>[6x]MCGRFLRRLLAEESRRSTPVGRLLLPVLLGFRLVLLAASGPGVYGDEQSEFVCHTQQPGCKAACFDAFHPLSPLRFWVFQVILVAVPSALYMGFTLYHVIWHWELSGKGKEEETLIQGREGNTDVPGAGSLRLLWAYVAQLGARLVLEGAALGLQYHLYGFQMPSSFACRREPCLGSITCNLSRPSEKTIFLKTMFGVSGFCLLFTFLELVLLGLGRWWRTWKHKSSSSKYFLTSESTRRHKKATDSLPVVETKEQFQEAVPGRSLAQEKQRPVGPRDA

Connexin family proteins assemble into hexameric channels called hemichannels/connexons, which function as transmembrane channels or dock together to form gap junction intercellular channels (GJIChs). Human Cx31.3/GJC3, which is expressed in oligodendrocytes of the central nervous systems, does not form intercellular channels. We determined the cryo–electron microscopy structures of human connexin 31.3 (Cx31.3)/GJC3 hemichannels in the presence and absence of calcium ions and with a hearing-loss mutation R15G at 2.3-, 2.5-, and 2.6-Å resolutions, respectively. We also found that the hemichannel has a pore with a diameter of ~8 Å and selectively transports chloride ions.

Six NTHs in the hemichannel are placed at the cytoplasmic entrance, whereas those in GJIChs are at the inner surface of the pore. The entrance-covering conformation appears to be stabilized mainly by intramolecular hydrophobic interactions of F5 and L9 in NTH, with T95, L96, V99, I100, and W103 in TM2. With this structure, we analyzed the solvent-accessible pore diameters along the pore axis and found that NTHs form the smallest pore with a diameter of ~8 Å, which is smaller than those of Cx26 (10 Å) and Cx46/50 (11 Å) GJICh structures. We identified long chains of map density on the hydrophobic surface, which likely correspond to lipid or detergent molecules. A strong density blob is located next to R144 in a deep hydrophilic pocket at the boundary of cytoplasmic and transmembrane regions, which spatially fit well at the head group of phosphatidylethanolamine (PE). In our putative PE-bound model, the phospho and amino groups of PE interact with the guanidino group of R144 and the carboxyl group of E13, respectively. In the Ca2+-free state, the tunnel is occupied by six water molecules (W1 to W6) with clear map densities, which form an extensive interaction network with the tunnel-lining residues. Therefore, we propose that the entrance-covering NTH conformation represents a partially closed state of Cx31.3 hemichannel, which would prevent the movement of metabolites through and selectively allows small anions to pass through the hemichannel.>[2x]PNSNATFNMELYNTDLFLVPSPGVFSV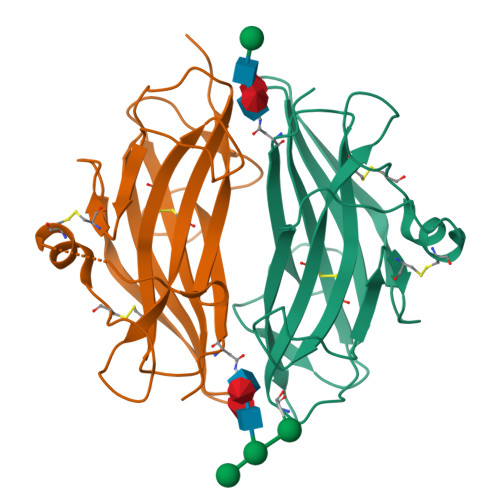AENEHVYVEVSVTKADQDLGFAIQTCFLSPYSNPDRMSDYTIIENICPKDDSVKFYSSKRVHFPIPHAEVDKKRFSFLFKSVFNTSLLFLHCELTLCSRKKGSLKLPRCVTPDDACTSLDATMIWTMMQNKKTFTKPLAVVLQVDYKEN> HHHHHHHHHHEQKLISEEDLDYKDDDDKMESEMLQSPLLGLGEEDEADLTDWNLPLAFMKKRHCEKIEGSKSLAQSWRMKDRMKTVSVALVLCLNVGVDPPDVVKTTPCARLECWIDPLSMGPQKALETIGANLQKQYENWQPRARYKQSLDPTVDEVKKLCTSLRRNAKEERVLFHYNGHGVPRPTVNGEVWVFNKNYTQYIPLSIYDLQTWMGSPSIFVYDCSNAGLIVKSFKQFALQREQELEVAAINPNHPLAQMPLPPSMKNCIQLAACEATELLPMIPDLPADLFTSCLTTPIKIALRWFCMQKCVSLVPGVTLDLIEKIPGRLNDRRTPLGELNWIFTAITDTIAWNVLPRDLFQKLFRQDLLVASLFRNFLLAERIMRSYNCTPVSSPRLPPTYMHAMWQAWDLAVDICLSQLPTIIEEGTAFRHSPFFAEQLTAFQVWLTMGVENRNPPEQLPIVLQVLLSQVHRLRALDLLGRFLDLGPWAVSLALSVGIFPYVLKLLQSSARELRPLLVFIWAKILAVDSSCQADLVKDNGHKYFLSVLADPYMPAEHRTMTAFILAVIVNSYHTGQEACLQGNLIAICLEQLNDPHPLLRQWVAICLGRIWQNFDSARWCGVRDSAHEKLYSLLSDPIPEVRCAAVFALGTFVGNSAERTDHSTTIDHNVAMMLAQLVSDGSPMVRKEL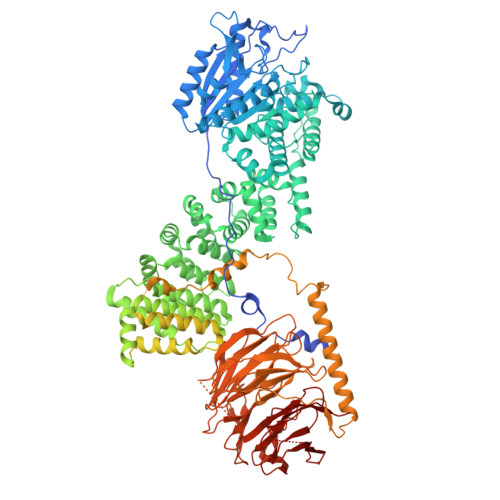VVALSHLVVQYESNFCTVALQFIEEEKNYALPSPATTEGGSLTPVRDSPCTPRLRSVSSYGNIRAVATARSLNKSLQNLSLTEESGGAVAFSPGNLSTSSSASSTLGSPENEEHILSFETIDKMRRASSYSSLNSLIGVSFNSVYTQIWRVLLHLAADPYPEVSDVAMKVLNSIAYKATVNARPQRVLDTSSLTQSAPASPTNKGVHIHQAGGSPPASSTSSSSLTNDVAKQPVSRDLPSGRPGTTGPAGAQYTPHSHQFPRTRKMFDKGPEQTADDADDAAGHKSFISATVQTGFCDWSARYFAQPVMKIPEEHDLESQIRKEREWRFLRNSRVRRQAQQVIQKGITRLDDQIFLNRNPGVPSVVKFHPFTPCIAVADKDSICFWDWEKGEKLDYFHNGNPRYTRVTAMEYLNGQDCSLLLTATDDGAIRVWKNFADLEKNPEMVTAWQGLSDMLPTTRGAGMVVDWEQETGLLMSSGDVRIVRIWDTDREMKVQDIPTGADSCVTSLSCDSHRSLIVAGLGDGSIRVYDRRMALSECRVMTYREHTAWVVKASLQKRPDGHIVSVSVNGDVRIFDPRMPESVNVLQIVKGLTALDIHPQADLIACGSVNQFTAIYNSSGELINNIKYYDGFMGQRVGAISCLAFHPHWPHLAVGSNDYYISVYSVEKRVR>TIPETPGPQFSQQREEDIYRFLKDNGPQRALVIAQALGMRTAKDV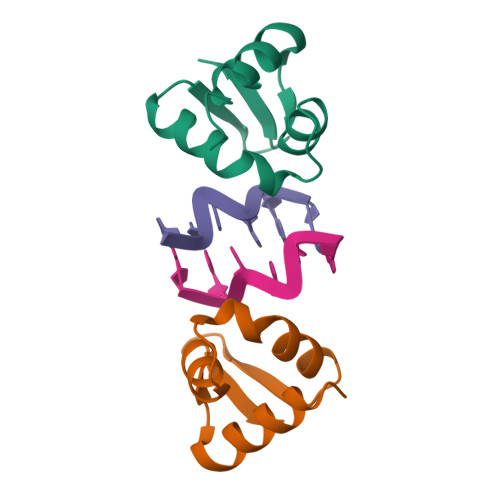NRDLYRMKSRHLLDMDEQSKAWTIY[4x]>[3x]MPEGPELHLASQFVNEACRALVFGGCVEKSSVSRNPEVPFESSAYRISASARGKELRLILSPLPGAQPQQEPLALVFRFGMSGSFQLVPREELPRHAHLRFYTAPPGPRLALCFVDIRRFGRWDLGGKWQPGRGPCVLQEYQQFRENVLRNLADKAFDRPICEALLDQRFFNGIGNYLRAEILYRLKIPPFEKARSVLEALQQHRPSPELTLSQKIRTKLQNPDLLELCHSVPKEVVQLGGRGYGSESPEEDFAAFRAWLRCYGMPGMSSLQDRHGRTIWFQGDPGPLAPKGRKS

Human endonuclease VIII-like 1 (hNEIL1) is a bifunctional DNA glycosylase of the Fpg/Nei family, which catalyzes the removal of damaged bases and subsequent incision of the newly generated abasic sites. Unlike traditional enzymes which are commonly referred to as highly specific biocatalysts, one special feature for hNEIL1 is its unique capability to recognize a wide range of substrates, including formamidopyrimidines, hydantoin lesions, oxidized, and dihydro-modified pyrimidine bases, derived from all four canonical bases. Here, by integrating structural, computational, and biochemical investigations, we show that hNEIL1 uses a triage mechanism to achieve broad specificity and reduce futile repair of normal bases. This mechanism involves two mutually competing interaction states: an activated state that commits catalysis and BER, and a quarantine state that temporarily separates and prevents the flipped base from catalysis via auto-inhibition.

We synthesized a 2′-fluoro-substituted stable mimic of DHU (FDHU), which allows binding but not catalysis by hNEIL1. In light of the observation that different hNEIL1–DNA interaction modes are largely resulted from the conformation changes of the lesion recognition loop, we chose to modify the potential key amino acids on this loop. In order to destabilize the quarantine state, we rationally designed hNEIL1(R242, G249P) and hNEIL1(R242, Y244H) to disrupt the flexibility of the loop or the aromatic stacking interactions respectively. Instead of the quarantine state originally observed in hNEIL1(R242)–FDHU structure, we found that both two mutants switched to the activated state as expected. Our study reveals that instead of utilizing a specific pocket to tightly recognize a flipped base via extensive electrostatic and hydrogen bonding interactions, hNEIL1 uses two competing interaction states to achieve substrate recognition. This mechanism is further corroborated by our finding that the relative dominance of the competing interaction states can be manipulated by artificially introduced or naturally existing mutations to the key lesion recognition loop.>[3x]QDEDAGGAGDETSEGEDTTGSDETPSTGGGGDGGNEETITAGNEDCWSKRPGWKLPDNLLTKTEFTSVDECRKMCEESAVEPSCYILQINTETNECYRNNEGDVTWSSLQYDQP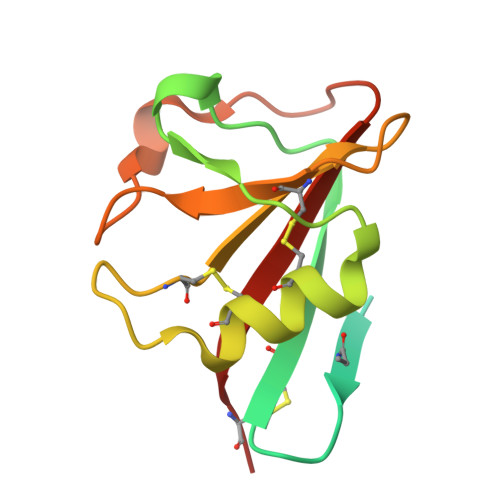NVVQWHLHACSK>MANDSPAKSLVDIDLSSLRDPAGIFELVEVVGNGTYGQVYKGRHVKTGQLAAIKVMDVTEDEEEEIKLEINMLKKYSHHRNIATYYGAFIKKSPPGHDDQLWLVMEFCGAGSITDLVKNTKGNTLKEDWIAYISREILRGLAHLHIHHVIHRDIKGQNVLLTENAEVKLVDFGVSAQLDRTVGRRNTFIGT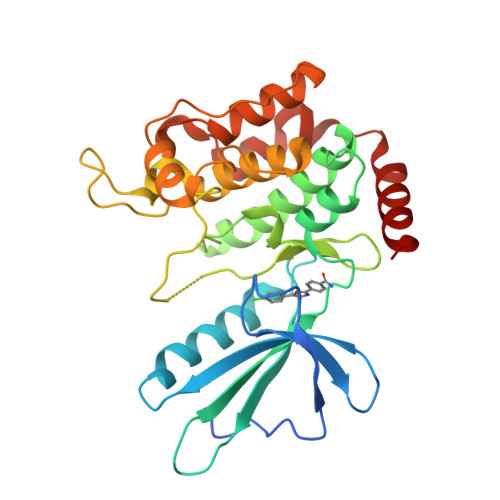PYWMAPEVIACDENPDATYDYRSDLWSCGITAIEMAEGAPPLCDMHPMRALFLIPRNPPPRLKSKKWSKKFFSFIEGCLVKNYMQRPSTEQLLKHPFIRDQPNERQVRIQLKDHIDRT[2x]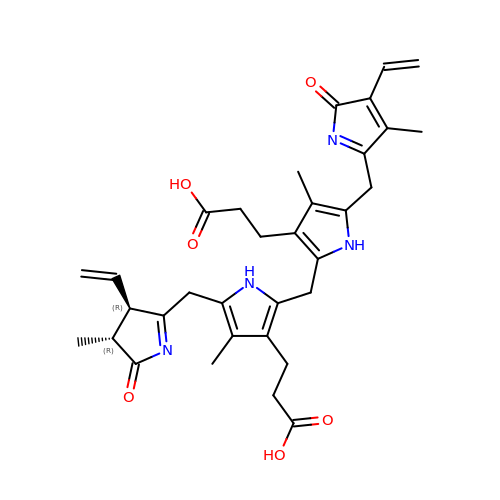3-[5-[[(3~{R},4~{R})-3-ethenyl-4-methyl-5-oxidanylidene-3,4-dihydropyrrol-2-yl]methyl]-2-[[5-[(4-ethenyl-3-methyl-5-oxidanylidene-pyrrol-2-yl)methyl]-3-(3-hydroxy-3-oxopropyl)-4-methyl-1~{H}-pyrrol-2-yl]methyl]-4-methyl-1~{H}-pyrrol-3-yl]propanoic acid | C33 H38 N4 O6 | IAVYOZQSRLDKLE-WOJBJXKFSA-N PUROMYCIN | C22 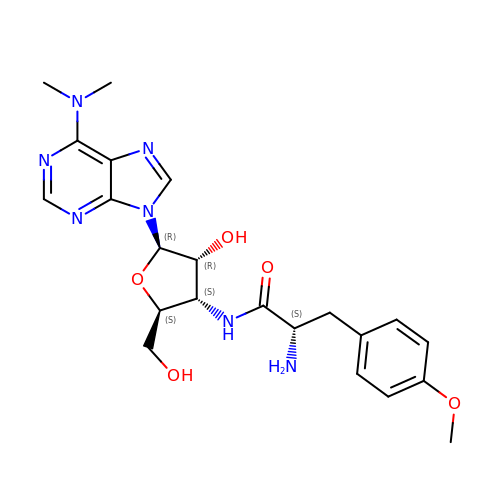H29 N7 O5 | RXWNCPJZOCPEPQ-NVWDDTSBSA-N>MFKMKVEDYFHDILRERKIHLTLIDPEEQTPEEAVEIARAAIRGGTDGIMLGGSTTDSSELDNTARALRENIDVPIILFPGNTTGVSRYADAIFFMSLLNSTNPYWIIGAQALGAATVKKMGIEALPMGYLVVEPGGTVGWVGDTKPVPRNKPDIAAAYAMEAEFLGMRLFYLEAGSGAPEHVPEEMIALVKRCTDQILIVGGGIRSGEDAARVAGAGADVVVTGTVVENSDNVEDKIREIVEGMGSVLEHHHHHH[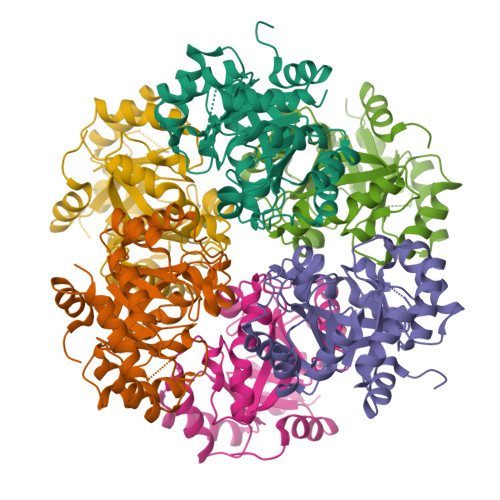6x]> HSQGTYTSDYSKYLDSRR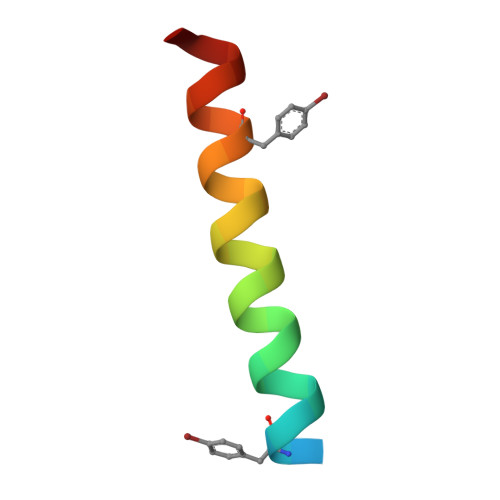AQDYVQWLMNT Pf4 and other Pf phages are members of the Inoviridae family which have recently been shown to be pervasive across all prokaryotes. Inoviruses are filamentous and rod-shaped, roughly six nm in diameter, that contain a single-stranded DNA (ssDNA) genome. Pf4 also promotes antibiotic tolerance of P. aeruginosa by self-assembling into higher-order liquid crystalline structures. The CoaB subunits adopt a 77-Å-long, α-helical structure, with the C-termini pointed toward the core of the phage and the N-termini directed toward the outside of the cylindrical filament.

We used real-space helical reconstruction to resolve a 3.2-Å resolution structure of the Pf4 phage. All side-chain densities for the 46-residue mature coat protein B (CoaB) of Pf4 are unambiguously assigned in our map. Pf4 filaments show a rise and rotation per subunit of 3.14 Å and 65.90°, respectively, allowing multiple CoaB molecules to pack tightly around the filament axis in an interdigitated array. The structure shows that Pf4 filaments have a diameter of ∼62 Å and an inner cavity with a diameter of ∼22 Å. Density for the ssDNA genome inside the 22-Å cavity in the core of the Pf4 phage is clearly resolved. Unexpectedly, this density shows that the Pf4 ssDNA genome is linear, rather than circular ssDNA, which was the expected paradigm for members of the Inoviridae family, since it was proposed for the related bacteriophage Pf1 (10) as well as fd. Clear density for the phosphate backbone of the ssDNA genome is resolved, but no density for a second antiparallel phosphate backbone is observed, as would be expected for circular ssDNA. The pitch of the linear ssDNA is 15.7 Å, meaning that there is exactly one CoaB protein for every base of ssDNA in the phage genome. Analysis of the interaction between CoaB protein subunits and the linear ssDNA genome (in the Pf4 structure with ssDNA) shows weak contacts between arginine 44 residues and the phosphate backbone of the DNA. The capsid coat itself is comparatively tightly packed, and is maintained by several hydrophobic interactions between the CoaB subunits, which repeat along the filament, likely providing large net stability to the phage structure.

> GVIDTSAVESAITDGQGDMKAIGGYIVGALVILAVAGLIYSMLRKA> HQSQLDRERILSLEQRVVELQQTLAQKDQALGKLEQSLRLMEEASFDGTFLWKITNVTRRCHESACGRTVSLFSPAFYTAKYGYKL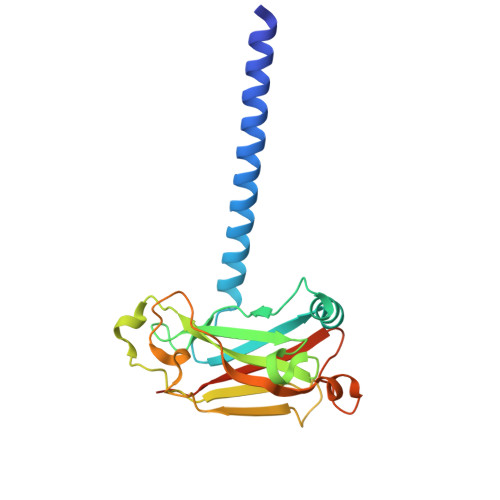CLRLYLNGDGTGKRTHLSLFIVIMRGEYDALLPWPFRNKVTFMLLDQNNREHAIDAFRPDLSSASFQRPQSETNVASGCPLFFPLSKLQSPKHAYVKDDTMFLKCIVETSTLEHHHHHH The human (h) TR exists in two isoforms, hTRα (NR1A1), and hTRβ (NR1A2). hTRα is expressed at higher levels in heart and plays a major role in regulation of heart rate, whereas TRβ is the predominant isoform that is expressed in the liver and pituitary and is involved with hepatic cholesterol metabolism and regulation of metabolic rate. Thyroid receptor (TR) activation occurs when an agonist ligand such as TH or similar compounds binds to a hydrophobic pocket in the core of its ligand-binding domain (LBD). This causes conformational changes which allow DNA bound receptors to interact with coactivators, mediating transcription.

Arg228 displays a double conformation in the first hTRα crystal form (P212121): a productive conformation identical to that of hTRβ and a non-productive conformation in which it points away from ligand (in green). No residues were observed in the disallowed regions of the plots, except for Arg188 in TRα structure in P212121. First, the GC-1 oxyacetic acid ester oxygen forms a hydrogen bond with the main chain amino group of TRα specific Ser277 residue. The Ser277 side chain hydroxyl participates in a hydrogen bond interaction with the Ile221 main chain carbonyl group, which is not available to Asn331 in hTRβ. This means that Ser277 fails to engage in a hydrogen bond contact with Arg228 analogous to that observed between Asn331 and Arg282. Thus, Arg228 is not anchored by contacts with the subtype specific residue. In addition, Ser277 is displaced by 1.64 Å toward the ligand compared to the T3-bound hTRα. This effect, coupled with the fact that dislocation and the smaller size of Ser relative to Asp in TRβ provides room for the Arg228 side chain to move, permits Arg228 to adopt apparent multiple conformations. In the productive conformation the ligand interacts strongly with the Arg228 residue and with the Ser277 by its oxyacetic oxygen. In the non-productive conformations GC-1 maintains the interaction with Ser277 but the strong interaction of GC-1 with Arg228 is lost, giving way to a hydrogen bond of this residue with the main carbonyl of Ser277. While hTRβ Arg282 binds to the ligand in a single conformation, hTRα Arg228 has the potential to flip away from the ligand in non-productive conformations, resulting in loss of an important interaction for the stabilization the ligand.

> GSHMEEMIRSLQQRPEPTPEEWDLIHIATEAHRSTNAQGSHWKQRRKFLPDDIGQSPIVSMPDGDKVDLEAFSEFTKIITPAITRVVDFAKKLPMFSELPCEDQIILLKGCCMEIMSLRAAVRYDPESDTLTLSGEMAVKREQLKNGGLGVVSDAIFELGKSLSAFNLDDTEVALLQAVLLMSTDRSGLLCVDKIEKSQEAYLLAFEHYVNHRKHNIPHFWPKLLMKVTDLRMIGACHASRFLHMKVECPTELFPPLFLEVFEDQEV>SKGLEDSSTISFITWNIDGLDGCNLPERARGVCSCLALYSPDVVFLQEVIPPYCAYLKKRAASYTIITGNEEGYFTAILLKKGRVKFKSQEIIPFPNTKMMRNLLCVNVSLGGNEFCLMTSHLESTREHSAERIRQLKTVLGKMQEAPDSTTVIFAGDTNLRDQEVIKCGGLPD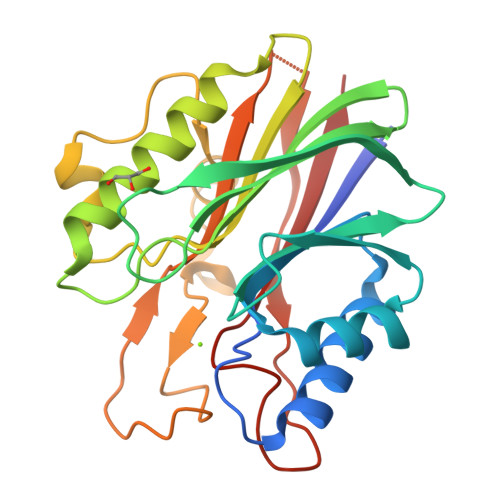NVFDAWEFLGKPKHCQYTWDTKANNNLRIPAAYKHRFDRIFFRAEEGHLIPQSLDLVGLEKLDCGRFPSDHWGLLCTLNVVL[5x]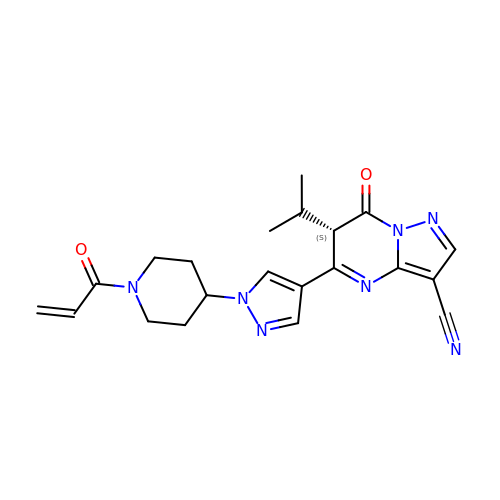7-oxidanylidene-6-propan-2-yl-5-[1-(1-prop-2-enoylpiperidin-4-yl)pyrazol-4-yl]-6~{H}-pyrazolo[1,5-a]pyrimidine-3-carbonitrile | C21 H23 N7 O2 | KGLWYCXNVRPKIE-SFHVURJKSA-N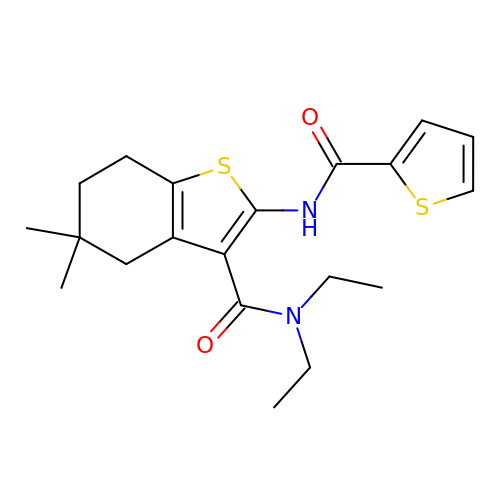N,N-DIETHYL-5,5-DIMETHYL-2-[(2-THIENYLCARBONYL)AMINO]-4,5,6,7-TETRAHYDRO-1-BENZOTHIOPHENE-3-CARBOXAMIDE | C20 H26 N2 O2 S2 | BCQPPORYBRTCLZ-UHFFFAOYSA-N> MELPGALQLGELAAAFASVPVFPL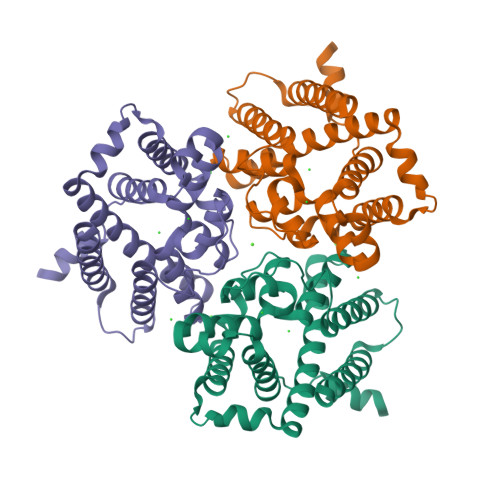FDAAYFIVSVLYLKYEPGAVEMSRKSPFASWLCAMLHCFGSYILADLLLGESPIHYFSNNSSVILATAVWYLIFFCPMNLFYKCVSFLPVKLIFVAMKEVVRVRAIAAGVHHAHHQYHHGWFIMMATGWVKGSGVALMSNFEQLLRGVWRPETNEILHMSFPTKASLYGTVLFTLQQTHWLPVSEANLVFFFTMFMIVCKVFMTATHSHASPFAPVEGFISPVFFGSVSSGHTSHHNQHGHSHEASYQPPPPVKSKEELNEGTRKRKAKKAEAAAENLYFQGLEDYKDDDDKHHHHHHHHHH>SNAMTNQDRPMKSMSESKCYKNRQVFPQDTNHHHTMFGGTLMANIDEIAAITAMKHAGAQVVTASTDSVDFLKPIKTGDILQYVAMVSYAGTSSMEVVVQIRIDDVFNNKHDLAALSYLTFVALDDEGKPKHVPGVYPEDDVEKW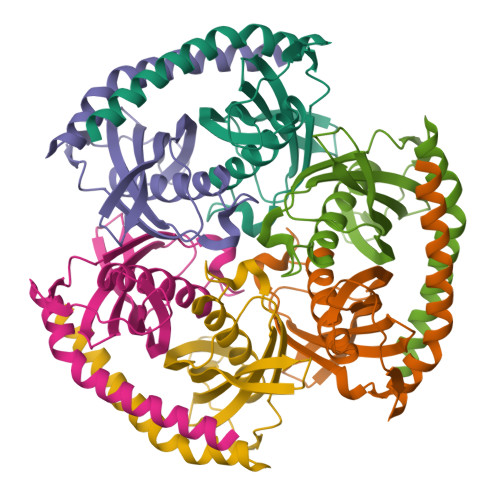FYDTAPQRVERRKARRIESKQTIEYLAQAQHIRD[6x]> MMRAAQKAKQELPATVLTQTRSYLAPLRSDFTEEITAPKVASASNLVNEWNNKKQATENLMKLLQAYKDIGDAKSEPLLKNHNPRTFEDRDYPVPDFRTQNLKAGDVPKFFDTVISTRASAAIASKDKFWAGRKTEAEAASAKASAAFPRVAVPEWKKGKTVSIENLNTVTDKYAAALVPKRKLALPVLPEGVKKAVEDFAASVGQAKNASEVSELLAKSLAEKAVVTEGGKVVEGFSYVSKAVAAKVIATRRAEVHERLLKLWAKRLLVSPELAIVPLNEF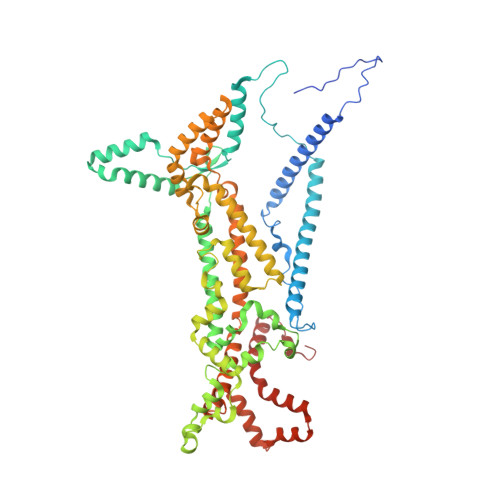DAQLASKFEGISPKYQELLSAVAQGNKTFAQRLNSSPAFSSFLLKREKAESEVPPSELELEAAQKAAELEDPEVALRTLLGPQMEALGASDLLLSEQIRVITEHRYTPDRLQYKEGMKLADKIAAQEAALKEELKVIYGDNVDVKHFQASPRTPVQQLFDSLKNAAANKERAAKEAAAAASPYLAYAVTKKQEVQADPSNIPFDEVLYPQLSEELLELELSDIREDEIALEKAEEEELWLLTLTQQFKHIQKHFGIDLPHSVVAHMDPLLIKKIDWETTNALEDFDITLDDMGAEDAKEQWGAENLSHHFLPLIRYRRDLARKNGDRYGPDLVNGN5-{(1R)-3-amino-4-fluoro-1-[3-(5-prop-1-yn-1-ylpyridin-3-yl)phenyl]-1H-isoindol-1-yl}-1-ethyl-3-methylpyridin-2(1H)-one 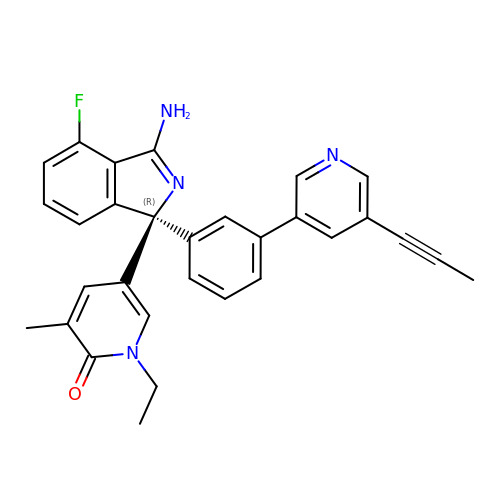| C30 H25 F N4 O | TUGLMYZSOPKJOA-PMERELPUSA-N>SNAMMEVCPYLEETFKILGRSWNGLIINYLSRSNDSSAHFSDMKRDLKTITPRALSLKLSELAQWELVEKQIISTSPVQIIYVLTEKGKAL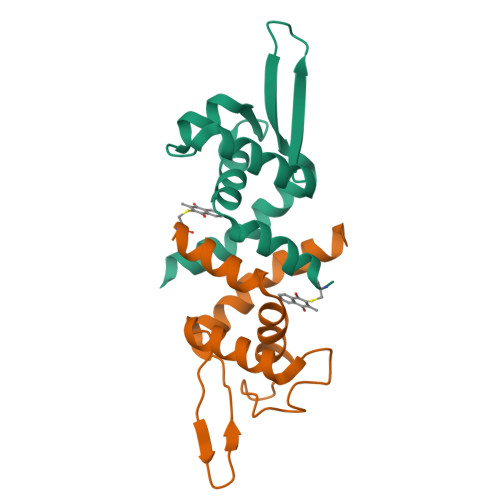AEALHPIEAWAQSYVDLTDQRTAK[2x]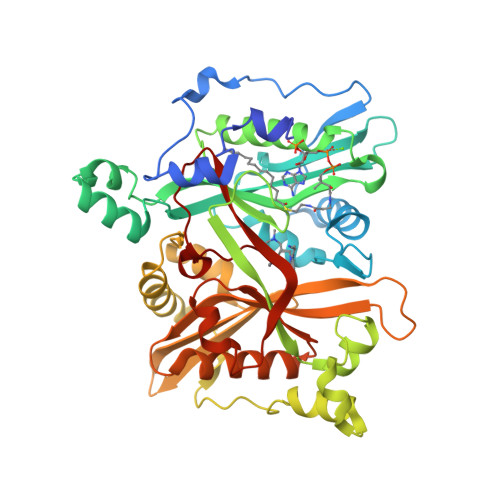> MSRNPSNSDAAHAFWSTQPVPQTEDETEKIVFAGPMDEPKTVADIPEEPYPIASTFEWWTPNMEAADDIHAIYELLRDNYVEDDDSMFRFNYSEEFLQWALCPPNYIPDWHVAVRRKADKKLLAFIAGVPVTLRMGTPKYMKVKAQEKGEGEEAAKYDEPRHICEINFLCVHKQLREKRLAPILIKEATRRVNRTNVWQAVYTAGVLLPTPYASGQYFHRSLNPEKLVEIRFSGIPAQYQKFQNPMAMLKRNYQLPSAPKNSGLREMKPSDVPQVRRILMNYLDSFDVGPVFSDAEISHYLLPRDGVVFTYVVENDKKVTDFFSFYRIPSTVIGNSNYNLLNAAYVHYYAATSIPLHQLILDLLIVAHSRGFDVCNMVEILDNRSFVEQLKFGAGDGHLRYYFYNWAYPKIKPSQVALVML>[2x]MFHSSAMVNSHRKPMFNIHRGFYCLTAILP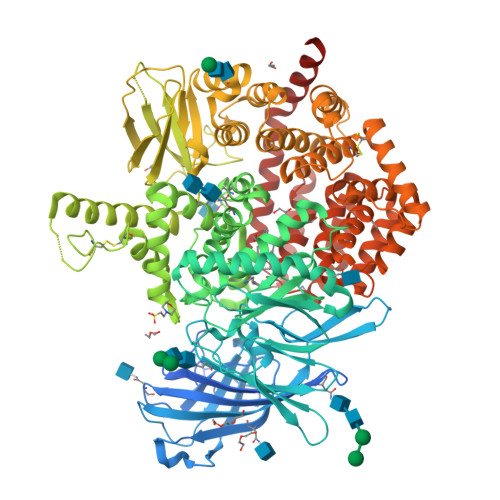QICICSQFSVPSSYHFTEDPGAFPVATNGERFPWQELRLPSVVIPLHYDLFVHPNLTSLDFVASEKIEVLVSNATQFIILHSKDLEITNATLQSEEDSRYMKPGKELKVLSYPAHEQIALLVPEKLTPHLKYYVAMDFQAKLGDGFEGFYKSTYRTLGGETRILAVTDFEPTQARMAFPCFDEPLFKANFSIKIRRESRHIALSNMPKVKTIELEGGLLEDHFETTVKMSTYLVAYIVCDFHSLSGFTSSGVKVSIYASPDKRNQTHYALQASLKLLDFYEKYFDIYYPLSKLDLIAIPDFAPGAMENWGLITYRETSLLFDPKTSSASDKLWVTRVIAHELAHQWFGNLVTMEWWNDIWLNEGFAKYMELIAVNATYPELQFDDYFLNVCFEVITKDSLNSSRPISKPAETPTQIQEMFDEVSYNKGACILNMLKDFLGEEKFQKGIIQYLKKFSYRNAKNDDLWSSLSNSCLESDFTSGGVCHSDPKMTSNMLAFLGENAEVKEMMTTWTLQKGIPLLVVKQDGCSLRLQQERFLQGVFQEDPEWRALQERYLWHIPLTYSTSSSNVIHRHILKSKTDTLDLPEKTSWVKFNVDSNGYYIVHYEGHGWDQLITQLNQNHTLLRPKDRVGLIHDVFQLVGAGRLTLDKALDMTYYLQHETSSPALLEGLSYLESFYHMMDRRNISDISENLKRYLLQYFKPVIDRQSWSDKGSVWDRMLRSALLKLACDLNHAPCIQKAAELFSQWMESSGKLNIPTDVLKIVYSVGAQTTAGWNYLLEQYELSMSSAEQNKILYALSTSKHQEKLLKLIELGMEGKVIKTQNLAALLHAIARRPKGQQLAWDFVRENWTHLLKKFDLGSYDIRMIISGTTAHFSSKDKLQEVKLFFESLEAQGSHLDIFQTVLETITKNIKWLEKNLPTLRTWLMVNTRH>DSISLSLINEGPSY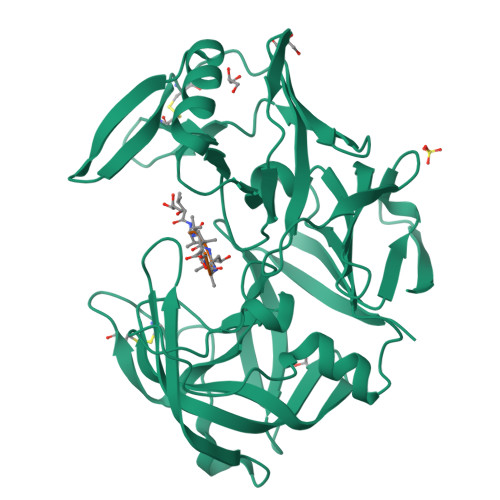ASKVSVGSNKQQQTVIIDTGSSDFWVVDSNAQCGKGVDCKSSGTFTPSSSSSYKNLGAAFTIRYGDGSTSQGTWGKDTVTINGVSITGQQIADVTQTSVDQGILGIGYTSNEAVYDTSGRQTTPNYDNVPVTLKKQGKIRTNAYSLYLNSPSAETGTIIFGGVDNAKYSGKLVAEQVTSSQALTISLASVNLKGSSFSFGDGALLDSGTTLTYFPSDFAAQLADKAGARLVQVARDQYLYFIDCNTDTSGTTVFNFGNGAKITVPNTEYVYQNGDGTCLWGIQPSDDTILGDNFLRHAYLLYNLDANTISIAQVKYTTDSSISAV[8x]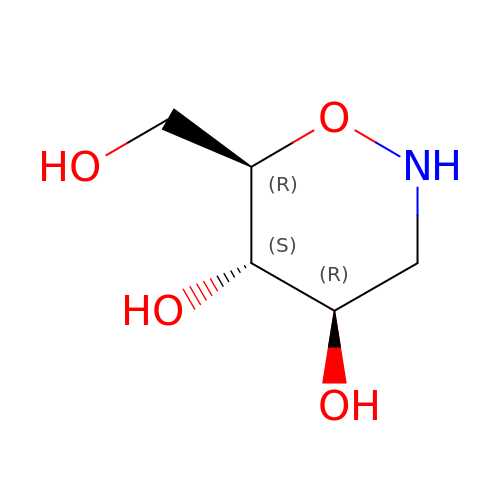TETRAHYDROOXAZINE | C5 H11 N O4 | KHVCOYGKHDJPBZ-WDCZJNDASA-N Many streptococci adhere to protein-attached carbohydrates expressed on cell surfaces using Siglec-like binding regions (SLBRs). Siglec-like binding regions (SLBRs) are among the streptococcal adhesive modules that bind sialoglycans. SLBRs contain two adjacent modules: a Siglec domain, which shares some features with mammalian Siglecs, and a Unique domain13 with no close homologs outside of the family. The conserved sialic acid-recognition motif governs general specificity while sequence diversity in surrounding loop regions allows the SLBR to select between related sialoglycans.

To understand selectivity of these SLBRs for human glycans, we chose comparators from each branch for detailed study. From the first branch of the tree (blue in Fig. 2), we selected the SLBRs of the Hsa adhesin from S. gordonii strain Challis (termed SLBRHsa) and the equivalent SLBRs from Streptococcus sanguinis strain SK678 (SLBRSK678) and Streptococcus gordonii strain UB10712 (SLBRUB10712; see footnote). Although these three SLBRs are >80% identical in amino acid sequence, when they were tested with arrays containing 49 sialoglycans, they exhibited distinct binding profiles. In comparison, SLBRUB10712 and SLBRSK678 were more narrowly selective, although both bound to multiple sialoglycan ligands. Specifically, SLBRUB10712 bound strongly to 3’-sialyl-N-acetyllactosamine (3’sLn; Neu5Acα2-3Galβ1-4GlcNAcβ, Fig. 1b) and a small range of related structures, while SLBRSK678 bound to only two of the glycans on this array, 3’sLn and 6-O-sulfo-sialyl Lewis X (6S-sLeX; Neu5Acα2-3Galβ1-4(Fucα1-3)GlcNAc6Sβ, Fig. 1c). To reveal how similar SLBRs could include or exclude different sialoglycans, we determined crystal structures of these five SLBRs at resolutions between 1.0 Å and 1.7 Å. We then evaluated selectivity conferred by the FG loop where crystallographic analysis would suggest that the β-branching of SLBRHsaD356 excludes C3 fucosylation, while the larger, unbranched Gln of SLBRUB10712 and SLBRSK678 can bind fucosylated ligands. Consistent with our prior studies, parent SLBRHsa preferentially bound proteoglycan 4 (460 kD) from human plasma, while SLBRUB10712 bound GPIbα (150 kD).

>[4x]GPGSNDTEAPQVKSGDYVVYRGESFEYYAEITDNSGQVNNVVVRNVELDKKTNMPYLTPDWLKYSTDNLGQPGNATVENPLRTKLYGNVPLDTVVGIYTRYIVATDPANNTTRMIQNPNRDGLERFVLTVKSQNEKYDPADPSVTYVNNLSNLSTSERDAVAAAVRAANPSLPSAAKITVSQNGTVTITYPDRSTDTIPANRVVKDLQIS1-[5-(4-fluoranyl-2-methyl-phenyl)-1~{H}-indazol-3-yl]-~{N},~{N}-dimethyl-methanamine | C17 H18 F N3 | 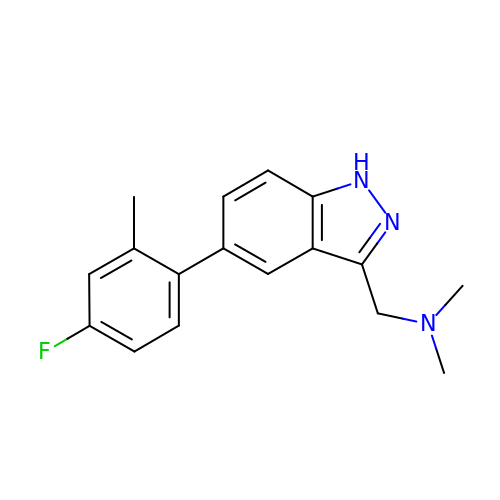DBUAKDPVYBEAFM-UHFFFAOYSA-N>MTTGLSTAGAQDIGRSSVRPYLEECTRRFQEMFDRHVVTRPTKVELTDAELREVIDDCNAAVAPLGKTVSDERWISYVGVVLWSQSPRHIKDMEAFKAVCVLNCVTFVWDDMDPALHDFGLFLPQLRKICEKYYGPEDAEVAYEAARAFVTSDHMFR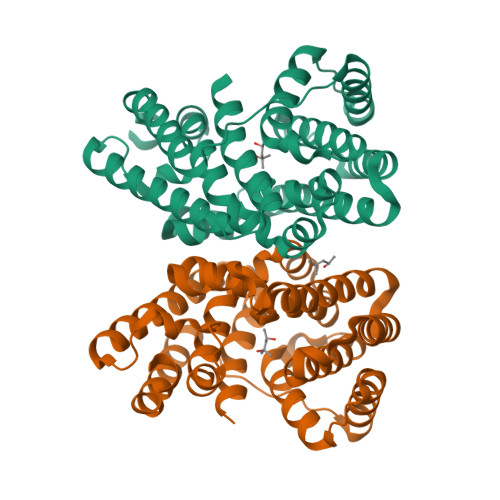DSPIKAALCTTSPEQYFRFRVTDIGVDFWMKMSYPIYRHPEFTEHAKTSLAARMTTRGLTIVNDFYSYDREVSLGQITNCFRLCDVSDETAFKEFFQARLDDMIEDIECIKAFDQLTQDVFLDLIYGNFVGTTSNKRYKTAVNDVNSRIQAAALEHHHHHH[2x]> SDRIIQITRGDSTITSQDVANAVVGYGVWPHYLTPQDATAIDKPTQPDTSSNRFYTLDSKMWNSTSKGWWWKLPDALKDMGIFGENMF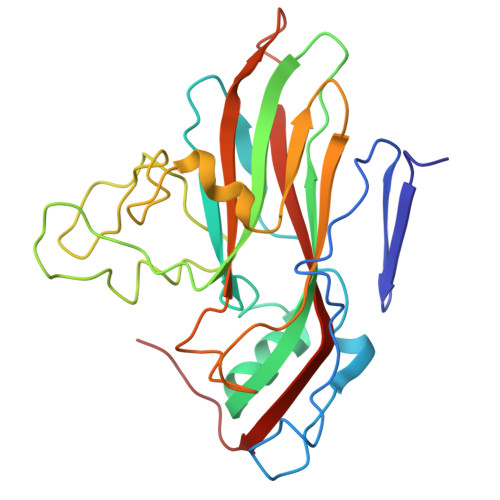YHFLGRSGYTVHVQCNASKFHQGTLLVVMIPEHQLATVNKGNVNAGYKYTHPGEAGREVGTAAAAEKQPSDDNWLNFDGTLLGNLLIFPHQFINLRSNNSATLIVPYVNAVPMDSMVRHNNWSLVIIPVCQLQSNNISNIVPITVSISPMCAEFSGARAKTVVQ(3~{S})-4-(4-hydroxyphenyl)-~{N}-oxidanyl-3-[5-[[(5-phenylthiophen-2-yl)sulfonylamino]methyl]-1,2,3-triazol-1-yl]butanamide 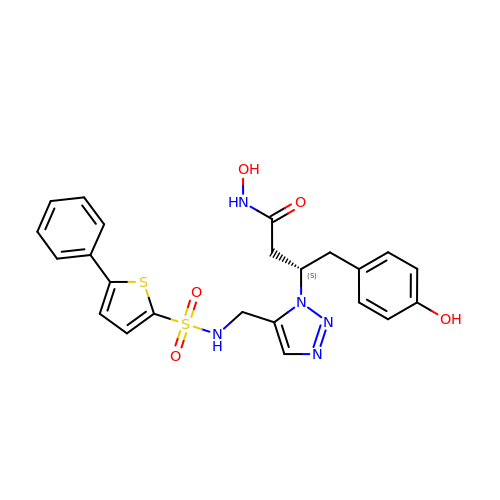| C23 H23 N5 O5 S2 | YNJVRCJGXCXRMB-SFHVURJKSA-N> MGSWEIDPKDLTFLKELGTGQFGVVKYGKWRGQY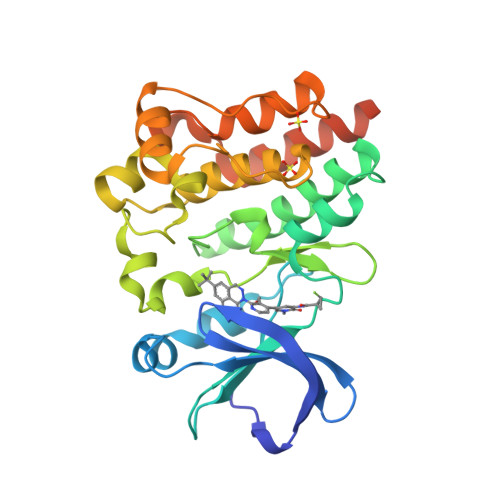DVAIKMIKEGSMSEDEFIEEAKVMMNLSHEKLVQLYGVCTKQRPIFIITEYMANGCLLNYLREMRHRFQTQQLLEMCKDVCEAMEYLESKQFLHRDLAARNCLVNDQGVVKVSDFGLSRYVLDDEYTSSVGSKFPVRWSPPEVLMYSKFSSKSDIWAFGVLMWEIYSLGKMPYERFTNSETAEHIAQGLRLYRPHLASEKVYTIMYSCWHEKADERPTFKILLSNILDVMDENLYFQGEEYMPTEHHHHHHHH>SEACAVHALFLILHSGNILDSGPGDANSKQADVQTLSSAFEAVTRIHFPEALGHVALRLVPCPPICAAAYALVSNLSPYSHDGDSLSRSQDHIPLAALPLLATSSSRYQGAVATVIARTNQAYSAFLRSPEGAGFCGQVALIGDGVGGILGFDALCHSANTARLDFKVSGFFLFGSPLGLVLALRKTVMPALEAAQMRPACEQIYNLFHAADPCASRLEPLLAPKFQAIAPLTVPRYQKFPLGDGSSLLLADTLQTHS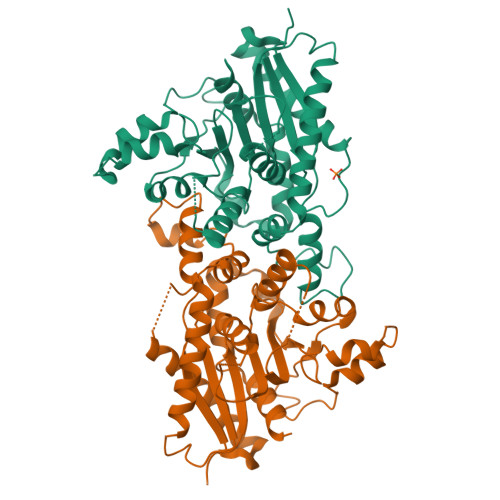SLFLEELEMLVPSTPTSTSGAFWKGSELATDPPAQPAAPSTTSEVVKILERWWGTKRIDYSLYCPEALTAFPTVTLPHLFHASYWESADVVAFILRQVIEKE[3x]>MADGQVAELLLRRLEASDGGLDSAELAAELGMEHQAVVGAVKSLQALGEVIEAELRSTKHWELTAEGEEIAREGSHEARVFRSIPPEGLAQSELMRLPSGKVGFSKAMSNKWIRVDKSAADGPRVFRVVDSMEDEVQRRLQLVRGGQAEKLGEKERSELRKRKLLAEVTLKTYWVSKGSAFSTSISKQETELSPEMISSGSWRDRPFKPYNFLAHGVLPDSGHLHPLLKVRSQFRQIFLEMGFTEMPTDNFIESSFWNFDALFQPQQHPARDQHDTFFLRDPAEALQLPMDYVQRVKRTHSQGGYGSQGYKYNWKLDEARKNLLRTHTTSASARALYRLAQKKPFTPVKYFSIDRVFRNETLDATHLAEFHQIEGVVADHGLTLGHLMG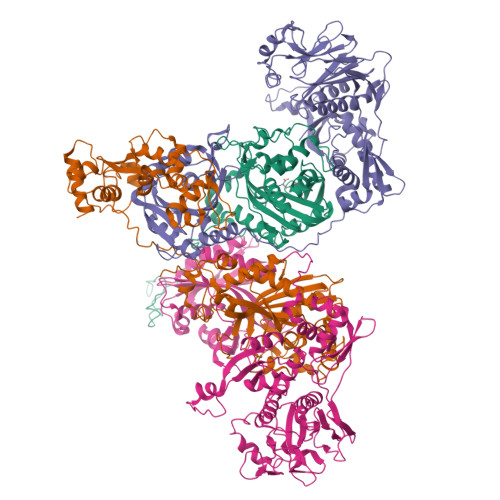VLREFFTKLGITQLRFKPAYNPYTEPSMEVFSYHQGLKKWVEVGNSGVFRPEMLLPMGLPENVSVIAWGLSLERPTMIKYGINNIRELVGHKVNLQMVYDSPLCRLDAEPRPPPTQEAA[8x];>[8x]MPTVSVKRDLLFQALGRTYTDEEFDELCFEFGLELDEITSEKEIISKEQGNVKAAGASDVVLYKIDVPANRYDLLCLEGLVRGLQVFKERIKAPVYKRVMPDGKIQKLIITEETAKIRPFAVAAVLRNIKFTKDRYDSFIELQEKLHQNICRKRALVAIGTHDLDTLSGPFTYTAKRPSDIKFKPLNKTKEYTACELMNIYKTDNHLKHYLHIIENKPLYPVIYDSNGVVLSMPPIINGDHSRITVNTRNIFIECTGTDFTKAKIVLDIIVTMFSEYCENQFTVEAAEVVFPNGKSHTFPELAYRKEMVRADLINKKVGIRETPENLAKLLTRMYLKSEVIGDGNQIEIEIPPTRADIIHACDIVEDAAIAYGYNNIQMTLPKTYTIANQFPLNKLTELLRHDMAAAGFTEALTFALCSQEDIADKLGVDISATKAVHISNPKTAEFQVARTTLLPGLLKTIAANRKMPLPLKLFEISDIVIKDSNTDVGAKNYRHLCAVYYNKNPGFEIIHGLLDRIMQLLDVPPGEDKGGYVIKASEGPAFFPGRCAEIFARGQSVGKLGVLHPDVITKFELTMPCSSLEINIGPFL>DADLAKKNNCIACHQVETKVVGPALKDIAAKYADKDDAATYLAGKIKGGSSGVWGQIPMPPVNVSDADAKALAD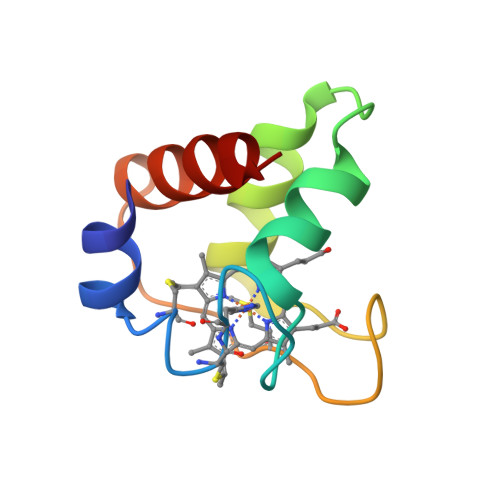WILTLK[4x]> MKNRLWLAMAAPLALATPVAFAQTPPTLAKDQAMPSLP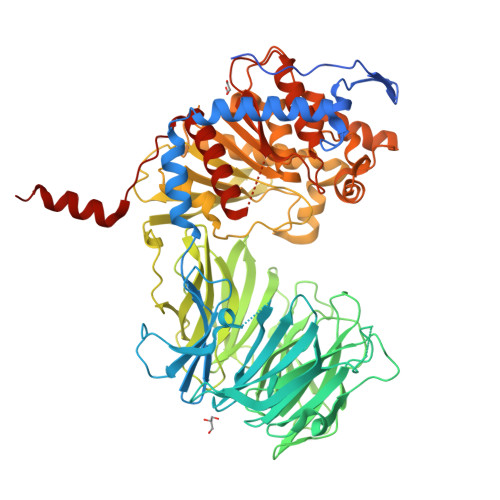PYPASPQVPLVEDHFGEKVSDPWRWLEADVRTDAKVAAWVQAQSAYTAAYLKQLPERAALEKRMKALIDYERFGLPQRRGASVFYSWNSGLMNQSQLLVRPADAPVGTKGRVLLDPNTWAKDGATALDAWAASDDGRLLAYSVQDGGSDWRTVKFVGVADGKPLADELKWVKFSGLAWLGNDALLYSRFAEPKEGQAFQALNYNQTVWLHRLGTPQSADQPVFATPELPKRGHGASVSSDGRWVVITSSEGTDPVNTVHVARVTNGKIGPVTALIPDLKAQWDFVDGVGDQLWFVSGDGAPLKKIVRVDLSGSTPRFDTVVPESKDNLESVGIAGNRLFASYIHDAKSQVLAFDLDGKPAGAVSLPGIGSASGLSGRPGDRHAYLSFSSFTQPATVLALDPATAKTTPWEPVHLTFDPADFRVEQVFYPSKDGTKVPMFIVRRKDAKGPLPTLLYGYGGFNVALTPWFSAGFMTWIDSGGAFALANLRGGGEYGDAWHDAGRRDKKQNVFDDFIAAGEWLIANGVTPRHGLAIEGGSNGGLLIGAVTNQRPDLFAAASPAVGVMDMLRFDQFTAGRYWVDDYGYPEKEADWRVLRRYSPYHNVRSGVDYPAILVTTADTDDRVVPGHSFKYTAALQTAAIGPKPHLIRIETRAGHGSGKPIDKQIEETADVQAFLAHFTGLTPRPWSSVDKLAAALEHHHHHH>MTTADRASEFLGGLFNSLTERGRSLFGLTSSQPMSGDELIALSETLLSRRGEASGVALAASLLAGYEAADEDDKLAFLDALAEQFGPDLAELNTAIEAFRADASAEATGELLRAAEPRRQELIRRLNHAPGGTAALVKMREAVLARIAAHPQLRHVDDDFVHLFTSWFNRGFLVLQRIDWTTPANILEKIIRYEQVHTIHDWDDLRARLAPPDRRCYGFFHPRLVDEPLIFVEVALTKDSPAAIAPLLDLEREPIAASDATTAVFYSISNTQQGLAGISFGNFLIKQVVEEIKRELPNVQTFVTLSPVPGFAKWLKRERDNPDSTLLDASARTALEALDTPNWFDDADTADRLKPIVLQLAAAYFLQAKGPNGRPLDPVARFHLGN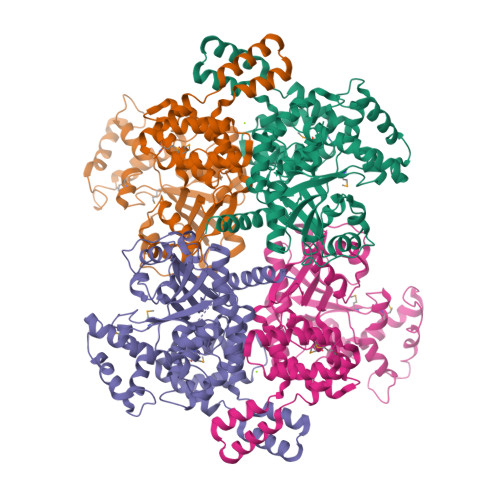GARLDRLNFLGDRSPNGMRQSHGLMVNYLYALGDIEANHEALFERGQIAAASAVRKLVPLEHHHHHH[4x]> MATEKKADVGKFVELPGAEMGKVIVRFPPEASGYLHIGHAKAALLNQ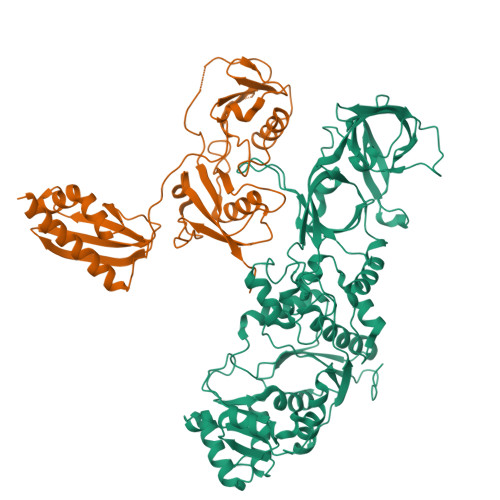HYQVNFKGKLIMRFDDTNPEKEKEDFEKVILEDVAMLHIKPDQFTYTSDHFETIMKYAEQLIQEGKAYVDDTPAEQMKAEREQRMESKHRNNCVNKNLQMWEEMKKGTEYGQTCCLRAKIDMNSNNGCMRDPTLYRCKNQPHPRTGTTYKVYPTYDFACPIVDSIEGVTHALRTTEYHDRDEQFYWIIEALGIRKPYIWEYSRLNLNNTVLSKRKLMWFVNEGLVDGWDDPRFPTVRGVLRRGMTVEGLKQFIAAQGSSRSVVNMEWDKIWSFNKKVIDPVAPRYTALLKDAVVPVNVPEAQEEMKEVAKHPKNADVGLKPVWYGSKVLIEGADAETLTEGEVVTFINWGNIIITKLNRNSSGKIVSIDTKLNLDNKDFKKTTKITWLAETPRAPLIPTVCVNYEHLITKPVLGKDEDFKQYINRNSKQEELMLGDPCLKDLKKGDIIQLQRRGFFICDQPYEPVSPYSCKEAPCILIYIPDGH;> HSDAQVLVLLDVTPDQSMVDEGVAREVINRIQKLRKKRNLVPTDEITVYYRSHPEGDYLDTVIKEHTDFIFATIKAALKPYPVPTSKEVLIQETTQLKGSELEITLVRGGLCERVGPACSYVNLKVCVNGTEQDGVLLLENPKGDNTLNLTGLVDAVSCIFGLKNSKLTVFNGKTELINKTDLLSLSGKTLHVTTGSAPALINSPDALLCQYINLQLVNAKPQECQKGTVGTLLMENPVGQNGLTYHGLLHETAKVFGLRSRRLKLFLDEAETQEITKDISMKNLNMKTVYVSVIPTTAEC> DMPVERILEAELAVEPKTETYVEANMGLNPSSPNDPVTNICQAADKQLFTLVEWAKRIPHFSELPLDDQVILLRAGWNELLIASFSHRSIAVKDGILLATGLHVH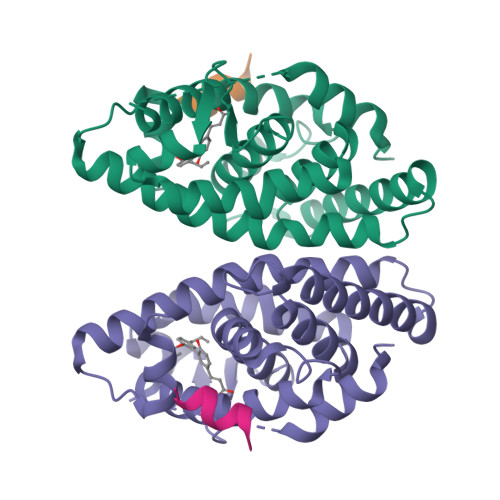RNSAHSAGVGAIFDRVLTELVSKMRDMQMDKTELGCLRAIVLFNPDSKGLSNPAEVEALREKVYASLEAYCKHKYPEQPGRFAKLLLRLPALRSIGLKCLEHLFFFKLIGDTPIDTFLMEMLEAP;> KILHRLLQD>[3x]SMPARIGYYEIDRTIGKGNFAVVKRATHLVTKAKVAIKIIDKTQLDEENLKKIFREVQIMKMLSHPHIIRLYQVMETERMIYLVTEYASGGEIFDHLV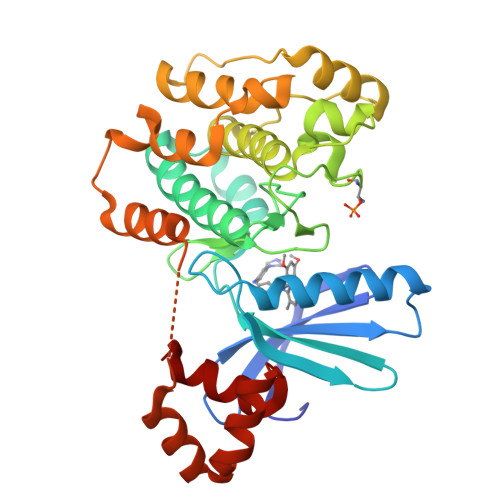AHGRMAEKEARRKFKQIVTAVYFCHSRNIVHRDLKAENLLLDANLNIKIADFGFSNLFTPGQLLKTWCGSPPYAAPELFEGKEYDGPKVDIWSLGVVLYVLVCGALPFDGSTLQNLRARVLSGKFRIPFFMSTECEHLIRHMLVLDPNKRLSMEQICKHKWMKLGDADPNFDRLIAESQQLKEERQVDPLNEDVLLAMEDMGLDKEQTLQSLRSDAYDHYSAIYSLLCDR> MDPDELPLDEHCERLPYDASKWEFPRDRLKLGKPLGRGAFGQVIEADAFGIDKTATCRTVAVKMLKEGATHSEHRALMSELKILIHIGHHLNVVNLLGACTKPGGPLMVIVEFCKFGNLSTYLRSKRNEFVPYKVAPEDLYKDFLTLEHLICYSFQVAKGMEFLASRKCIHRDLAARNILLSEKNVVK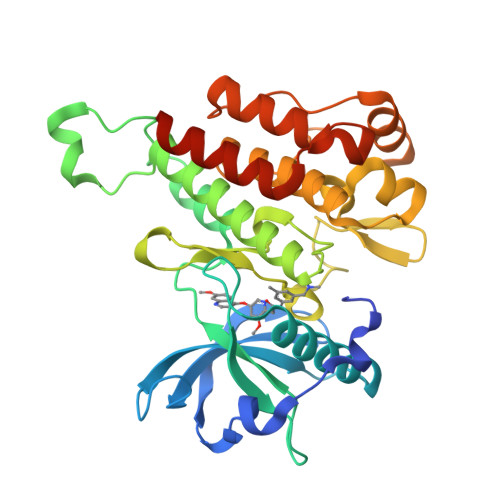ICDFGLARDIYKDPDYVRKGDARLPLKWMAPETIFDRVYTIQSDVWSFGVLLWEIFSLGASPYPGVKIDEEFCRRLKEGTRMRAPDYTTPEMYQTMLDCWHGEPSQRPTFSELVEHLGNLLQANAQQDENLYFQ> MLRTMLKSKIHRATVTCADLHYVG;> XVTIDADLMDAADLLEGEQVTIVDIDNGARLVTYAITGERGSGVIGINGAAAHLVHPGDLVILIAYATMDDARARTYQPRIVFVDAYNKPIDIGHD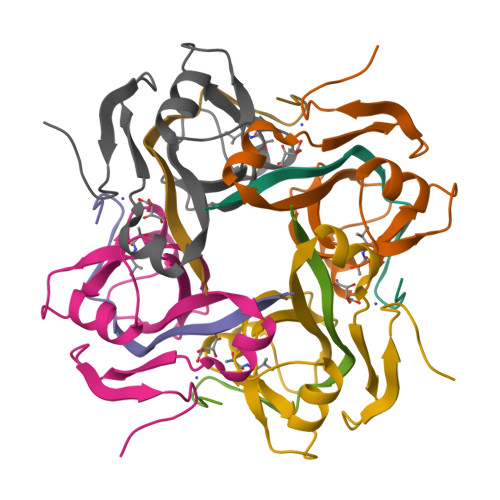PAFVPENAGELLDPRLGVGLEHHHHHH>MDTEGFGELLQQAEQLAAETEGISELPHVERNLQEIQQAGERLRSRTLTRTSQETADVKASVLLGSRGLDISHISQRLESLSAATTFEPLEPVKDTDIQGFLKNEKDNALLSAIEESRKRTFGMAEEYHRESMLVEWEQVKQRILHTLLASGEDALDFTQESEPSYISDVGPPGRSSLDNIEMAYARQIYIYNEKIVNGHLQPNLVDLCASVAELDDKSISDMWTMVKQMTDVLLTPATDALKNRSSVEVRMEFVRQALAYLEQSYKNYTLVTVFGNLHQAQLGGVPGTYQLVRSFLNIKLPAPLPGLQDGEVEGHPVWALIYYCMRCGDLLAASQVVNRAQHQLGEFKTWFQEYMNSKDRRLSPATENKLRLHYRRALRNNTDPYKRAVYCIIGRCDVTDNQSEVADKTEDYLWLKLNQVCFDDDGTSSPQDRLTLSQFQKQLLEDYGESHFTVNQQPFLYFQVLFLTAQFEAAVAFLFRMERLRCHAVHVALVLFELKLLLKSSGQSAQLLSHEPGDPPCLRRLNFVRLLMLYTRKFESTDPREALQYFYFLRDEKDSQGENMFLRCVSELVIESREFDMILGKLENDGSRKPGVIDKFTSDTKPIINKVASVAENKGLFEEAAKLYDLAKNADKVLELMNKLLSPVVPQISAPQSNKERLKNMALSIAERYRAQGISANKFVDSTFYLLLDLITFFDEYHSGHIDRAFDIIERLKLVPLNQESVEERVAAFRNFSDEIRHNLSEVLLATMNILFTQFKRLKGTSPSSSSRPQRVIEDRDSQLRSQARTLITFAGMIPYRTSGDTNARLVQMEVLMN[4x];>MATPLAVNSAASLWGPYKDIWHKVGNALWRRQPEAVHLLDKILKKHKPDFISLFKNPPKNVQQHEKVQKASTEGVAIQGQQGTRLLPEQLIKEAFILSDLFDIGELAAVELLLAGEHQQPHFPGLTRGLVAVLLYWDGKRCIANSLKALIQSRRGKTWTLELSPELASMTTRFTDELMEQGLTYKVLTLVSQIDVNNEFEKLQRERGLGSEKHRKEVSDLIKECRQSLAESLFAWACQSPLGKEDTLLLIGHLERVTVEANGSLDAVNLALLMALLYCFDISFIEQSTEERDDMIHQLPLLTEKQYIATIHSRLQDSQLWKLPGLQATVRLAWALALRGISQLPDVTALAEFTEADEAMAELAIADNVFLFLMESVVVSEYFYQEEFYIRRVHNLITDFLALMPMKVKQLRNRADEDARMIHMSMQMGNEPPISLRRDLEHLMLLIGELYKKNPFHLELALEYWCPTEPLQTPTIMGSYLGVAHQRPPQRQVVLSKFVRQMGDLLPPTIYIPYLKMLQGLANGPQCAHYCFSLLKVNGSSHVENIQGAGGSPVSWEHFFHSLMLYHEHLRKDLPSADSVQYRHLPSRGITQKEQDGLIAFLQLTSTIITWSENARLALCEHPQWTPVVVILGLLQCSIPPVLKAELLKTLAAFGKSPEIAASLWQSLEYTQILQTVRIPSQRQAIGIEVELNEIESRCEEYPLTRAFCQLISTLVESSFPSNLGAGLRPPGFDPYLQFLRDSVFLRFRTRAYRRAAEKWEVAEVVLEVFYKLLRDYEPQLEDFVDQFVELQGEEIIAYKPPGFSLMYHLLNESPMLELALSLLEEGVKQLDTYAPFPGKKHLEKAVQHCLALLNLTLQKENLFMDLLRESQLALIVCPLEQLLQGINPRTKKADNVVNIARYLYHGNTNPELAFESAKILCCISCNSNIQIKLVGDFTHDQSISQKLMAGFVECLDCEDAEEFVRLEEGSELEKKLVAIRHETRIHILNLLITSLECNPPNLALYLLGFELKKPVSTTNLQDPGVLGCPRTCLHAILNILEKGTEGRTGPVAVRESPQLAELCYQVIYQLCACSDTSGPTMRYLRTSQDFLFSQLQYLPFSNKEYEISMLNQMSWLMKTASIELRVTSLNRQRSHTQRLLHLLLDDMPVKPYSDGEGGIEDENRSVSGFLHFDTATKVRRKILNILDSIDFSQEIPEPLQLDFFDRAQIEQVIANCEHKNLRGQTVCNVKLLHRVLVAEVNALQGMAAIGQRPLLMEEISTVLQYVVGRNKLLQCLHAKRHALESWRQLVEIILTACPQDLIQAEDRQLIIRDILQDVHDKILDDEAAQELMPVVAGAVFTLTAHLSQAVLTEQKETSVLGPAEAHYAFMLDSCFTSPPPEENPLVGFASIGDSSLYIILKKLLDFILKTGGGFQRVRTHLYGSLLYYLQIAQRPDEPDTLEAAKKTMWERLTAPEDVFSKLQRENIAIIESYGAALMEVVCRDACDGHEIGRMLALALLDRIVSVDKQQQWLLYLSNSGYLKVLVDSLVEDDRTLQSLLTPQPPLLKALYTYESKMAFLTRVAKIQQGALELLRSGVIVRLAQCQVYDMRPETDPQSMFGMRDPPMFIPTPVDRYRQILLPALQLCQVILTSSMAQHLQAAGQVLQFLISHSDTIQAILRCQDVSAGSLQELALLTGIISKAALPGILSELDVDVNEGSLMELQGHIGRFQRQCLGLLSRFGGSDRLRQFKFQDDNVEGDKVSKKDEIELAMQQICANVMEYCQSLMLQSSPTFQHAVCLFTPSLSETVNRDGPRQDTQAPVVPYWRLPGLGIIIYLLKQSANDFFSYYDSHRQSVSKLQNVEQLPPDEIKELCQSVMPAGVDKISTAQKYVLARRRLVKVINNRAKLLSLCSFIIETCLFILWRHLEYYLLHCMPTDSQDSLFASRTLFKSRRLQDSFASETNLDFRSGLAIVSQHDLDQLQADAINAFGESLQKKLLDIEGLYSKVRSRYSFIQALVRRIRGLLRISRN[4x];>MPSSLLGAAMPASTSAAALQEALENAGRLIDRQLQEDRMYPDLSELLMVSAPNNPTVSGMSDMDYPLQGPGLLSVPNLPEISSIRRVPLPPELVEQFGHMQCNCMMGVFPPISRAWLTIDSDIFMWNYEDGGDLAYFDGLSETILAVGLVKPKAGIFQPHVRHLLVLATPVDIVILGLSYANLQTGSGVLNDSLSGGMQLLPDPLYSLPTDNTYLLTITSTDNGRIFLAGKDGCLYEVAYQAEAGWFSQRCRKINHSKSSLSFLVPSLLQFTFSEDDPILQIAIDNSRNILYTRSEKGVIQVYDLGQDGQGMSRVASVSQNAIVSAAGNIARTIDRSVFKPIVQIAVIENSESLDCQLLAVTHAGVRLYFSTCPFRQPLARPNTLTLVHVRLPPGFSASSTVEKPSKVHRALYSKGILLMAASENEDNDILWCVNHDTFPFQKPMMETQMTAGVDGHSWALSAIDELKVDKIITPLNKDHIPITDSPVVVQQHMLPPKKFVLLSAQGSLMFHKLRPVDQLRHLLVSNVGGDGEEIERFFKLHQEDQACATCLILACSTAACDREVSAWATRAFFRYGGEAQMRFPTTLPPPSNVGPILGSPVYSSSPVPSGSPYPNPSFLGTPSHGIQPPAMSTPVCALGNPATQATNMSCVTGPEIVYSGKHNGICIYFSRIMGNIWDASLVVERIFKSGNREITAIESSVPCQLLESVLQELKGLQEFLDRNSQFAGGPLGNPNTTAKVQQRLIGFMRPENGNPQQMQQELQRKFHEAQLSEKISLQAIQQLVRKSYQALALWKLLCEHQFTIIVAELQKELQEQLKITTFKDLVIRDKELTGALIASLINCYIRDNAAVDGISLHLQDICPLLYSTDDAICSKANELLQRSRQVQNKTEKERMLRESLKEYQKISNQVDLSNVCAQYRQVRFYEGVVELSLTAAEKKDPQGLGLHFYKHGEPEEDIVGLQAFQERLNSYKCITDTLQELVNQSKAAPQSPSVPKKPGPPVLSSDPNMLSNEEAGHHFEQMLKLSQRSKDELFSIALYNWLIQVDLADKLLQVASPFLEPHLVRMAKVDQNRVRYMDLLWRYYEKNRSFSNAARVLSRLADMHSTEISLQQRLEYIARAILSAKSSTAISSIAADGEFLHELEEKMEVARIQLQIQETLQRQYSHHSSVQDAVSQLDSELMDITKLYGEFADPFKLAECKLAIIHCAGYSDPILVQTLWQDIIEKELSDSVTLSSSDRMHALSLKIVLLGKIYAGTPRFFPLDFIVQFLEQQVCTLNWDVGFVIQTMNEIGVPLPRLLEVYDQLFKSRDPFWNRMKKPLHLLDCIHVLLIRYVENPSQVLNCERRRFTNLCLDAVCGYLVELQSMSSSVAVQAITGNFKSLQAKLERLH[4x];>MAFNFGAPSGTSGTAAATAAPAGGFGGFGTTSTTAGSAFSFSAPTNTGTTGLFGGTQNKGFGFGTGFGTTTGTSTGLGTGLGTGLGFGGFNTQQQQQTTLGGLFSQPTQAPTQSNQLINTASALSAPTLLGDERDAILAKWNQLQAFWGTGKGYFNNNIPPVEFTQENPFCRFKAVGYSCMPSNKDEDGLVVLVFNKKETEIRSQQQQLVESLHKVLGGNQTLTVNVEGTKTLPDDQTEVVIYVVERSPNGTSRRVPATTLYAHFEQANIKTQLQQLGVTLSMTRTELSPAQIKQLLQNPPAGVDPIIWEQAKVDNPDSEKLIPVPMVGFKELLRRLKVQDQMTKQHQTRLDIISEDISELQKNQTTSVAKIAQYKRKLMDLSHRTLQVLIKQEIQRKSGYAIQADEEQLRVQLDTIQGELNAPTQFKGRLNELMSQIRMQNHFGAVRSEERYYIDADLLREIKQHLKQQQEGLSHLISIIKDDLEDIKLVEHGLNETIHIRGGVFS[4x];>MSTGFSFGSGTLGSTTVAAGGTSTGGVFSFGTGASSNPSVGLNFGNLGSTSTPATTSAPSSGFGTGLFGSKPATGFTLGGTNTGIATTITTGLTLGTPATTSAATTGFSLGFNKPAASATPFALPITSTSASGLTLSSALTSTPAASTGFTLNNLGGTTATTTTASTGLSLGGALAGLGGSLFQSTNTGTSGLGQNALGLTLGTTAATSTAGNEGLGGIDFSSSSDKKSDKTGTRPEDSKALKDENLPPVICQDVENLQKFVKEQKQVQEEISRMSSKAMLKVQEDIKALKQLLSLAANGIQRNTLNIDKLKIETAQELKNAEIALRTQKTPPGLQHEYAAPADYFRILVQQFEVQLQQYRQQIEELENHLATQANNSHITPQDLSMAMQKIYQTFVALAAQLQSIHENVKVLKEQYLGYRKMFLGDAVDVFETRRAEAKKWQNTPRVTTGPTPFSTMPNAAAVAMAATLTQQQQPATGPQPSLGVSFGTPFGSGIGTGLQSSGLGSSNLGGFGTSSGFGCSTTGASTFGFGTTNKPSGSLSAGFGSSSTSGFNFSNPGITASAGLTFGVSNPASAGFGTGGQLLQLKKPPAGNKRGKR[4x];>MSGFNFGGTGAPTGGFTFGTAKTATTTPATGFSFSTSGTGGFNFGAPFQPATSTPSTGLFSLATQTPATQTTGFTFGTATLASGGTGFSLGIGASKLNLSNTAATPAMANPSGFGLGSSNLTNAISSTVTSSQGTAPTGFVFGPSTTSVAPATTSGGFSFTGGSTAQPSGFNIGSAGNSAQPTAPATLPFTPATPAATTAGATQPAAPTPTATITSTGPSLFASIATAPTSSATTGLSLCTPVTTAGAPTAGTQGFSLKAPGAASGTSTTTSTAATATATTTSSSSTTGFALNLKPLAPAGIPSNTAAAVTAPPGPGAAAGAAASSAMTYAQLESLINKWSLELEDQERHFLQQATQVNAWDRTLIENGEKITSLHREVEKVKLDQKRLDQELDFILSQQKELEDLLSPLEELVKEQSGTIYLQHADEEREKTYKLAENIDAQLKRMAQDLKDIIEHLNTSGAPADTSDPLQQICKILNAHMDSLQWIDQNSALLQRKVEEVTKVCEGRRKEQERSFRITFD[4x]

Nuclear pore complexes (NPCs) create large conduits for cargo transport between the nucleus and cytoplasm across the nuclear envelope (NE). These multi-megadalton structures are composed of about thirty different nucleoporins that are distributed in three main substructures (the inner, cytoplasmic and nucleoplasmic rings) around the central transport channel. Here we use cryo-electron tomography on DLD-1 cells that were prepared using cryo-focused-ion-beam milling to generate a structural model for the human NPC in its native environment. Our findings highlight the inherent flexibility of the NPC and suggest that the cellular environment has a considerable influence on NPC dimensions and architecture.

The inner ring (IR) is centrally positioned at the fusion point of the inner and outer nuclear membranes (INM and ONM, respectively) and forms the central channel that connects to phenylalanine–glycine (FG) repeat proteins that create the permeability barrier and facilitate active cargo transport. FG-Nups (Nup54, Nup58 and Nup62) are docked to the IR to create the central channel for transport. For the IR, we first docked the published composite model containing Nup93, Nup188/Nup205, Nup155 and the Nup62–Nup58–Nup54 complex9. Although this model fits well, some elements appear to be shifted, suggesting that flexibility in the IR Nups may account for the larger diameter that we observed. To better fit the model, we isolated individual Nups and reoriented them locally to create an updated IR model. In our IR model, Nup205/Nup188 (paralogues that are indistinguishable at this resolution), Nup155 and Nup93 are significantly shifted, whereas the Nup62–Nup58–Nup54 complex is stable. Propagated through the entire IR, these rearrangements explain how the central channel becomes larger. The Nup93 and Nup205 subunits of adjacent IR structures form a pseudo-lock-and-key configuration in the constricted IR model; by contrast, here these components shifted to create gaps between the IR subunits. Adjacent IR subunits are nearly separated compared with previous models in which the subunits were snugly aligned. However, the diameter of the central channel is considerably different —it is about 33% larger (width, about 57 nm) compared with previous models (width, about 43 nm).>GPLGSPQFMNPAAEAEFNILLATDSYKVTHYKQYPPNTSKVYSYFECREKKTENSKLRKVKYEETVFYGLQYILNKYLKGKVVTKEKIQEAKDVYKEHFQDDVFNEKGWNYILEKYDGHLPIEIKAVPEGFVIPRGNVLFTVENTDPECYWLTNWIETILVQSWYPITVATNSREQKKILAKYLLETSGNLDGLEYKLHDFGYRGVSSQETAGIGASAHLVNFKGTDTVAGLALIKKYYGTKDPVPGYSVPAAEHSTITAWGKDHEKDAFEHIVTQFSSVPVSVVSDSYDIYNACEKIWGEDLRHLIVSRSTQAPLIIRPDSGNPLDTVLKVLEILGKKFPVTENSKGYKLLPPYLRVIQGDGVDINTL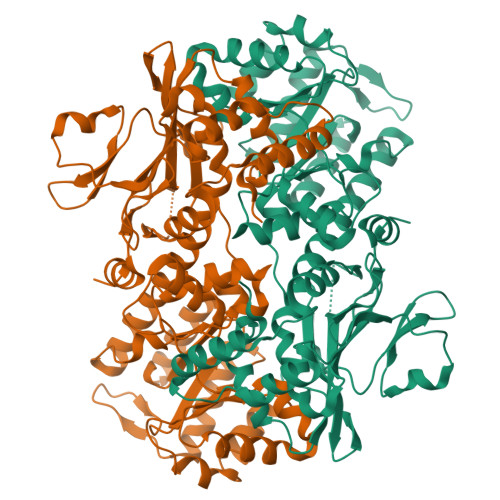QEIVEGMKQKMWSIENIAFGSGGGLLQKLTRDLLNCSFKCSYVVTNGLGINVFKDPVADPNKRSKKGRLSLHRTPAGNFVTLEEGKGDLEEYGQDLLHTVFKNGKVTKSYSFDEIRKNAQLNIELEAAHH[2x]>MTNLPTALITGASSGIGATYAERFARRGHNLVMVARDKVRMDVLASRLREETKVTIDVIQADLTQQKDLAEVETRLR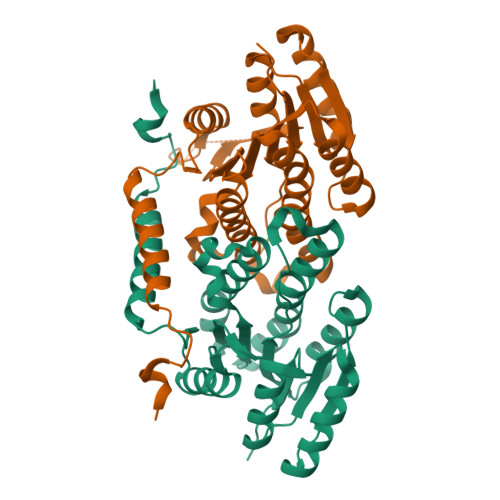EDTSIGILINNAGMGQSGAFVQQNAQSIDRLVMLNTTAPTRLAAAVAARFAQEGKGSIVNIGSVVGFAPELGMTIYGATKAFVLFLSQGLNLELGPKGIYVQAVLPAATRTEIWSRAGMDINTLPEVMDVNELVDAALIGFDRKELVTIPPLHVAERWNELDQARQGLMSEIRQAHAAERYLPQALEHHHHHH[3x]>[2x]HGGVLAYSLAGTWYNGFVPYNTPTGQSTIQREWDTYNPITDPTDASISCNINGASLGSAQK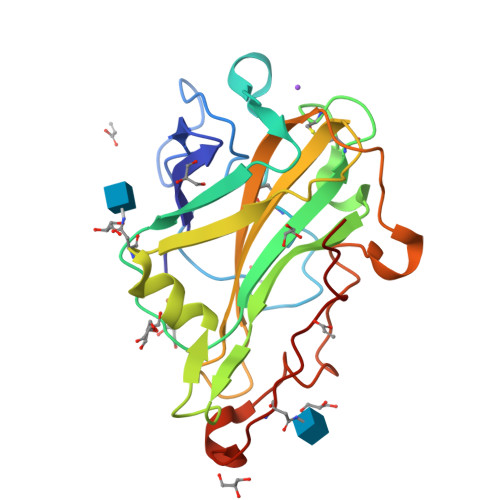SATVAAGSSVTAYWNQWPHTIGPVMVYMANCGGDCTTATTSSLEWFKINQVGLVSGTLTSGTWGMGQLVANNNSWTTSIPSSLAAGNYILRHELLAIHTSNQPQFYPECAQLIVTGGEGATPPASYLVKLPGAYSMSDPGVNIDIYSHETETNYTIPGPAVWQG>QFYSSLIEEIGTLGWDKLVYADTCFSTIKLKAEDASGREHLITLKLKAKYPAESPDYFVDFPVPFCASWTPQSSLISIYSQFLAAIESLKAFWDVMDEIDEKTWVLEPEKPPRSATARRIALGNNVSINIEVDPRHPTMLPECF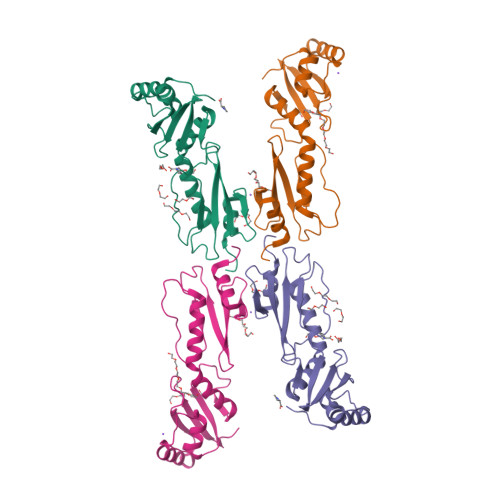FLGADHVVKPLGIKLSRNIHLWDPENSVLQNLKDVLEIDFPA[2x]> MEEPEEPADSGQSLVPVYIYSPEYVSMCDSLAKIPKRASMVHSLIEAYALHKQMRIVKPKVASMEEMATFHTDAYLQHLQKVSQEGDDDHLDSIEYGLGYDCPATEGIFDYAAAIGGAT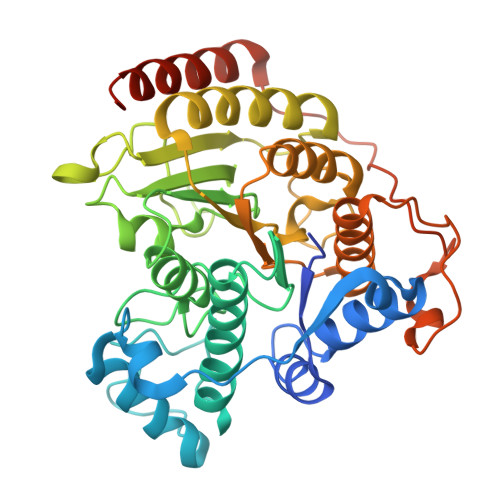ITAAQCLIDGMCKVAINWSGGWHHAKKDEASGFCYLNDAVLGILRLRRKFERILYVDLDLHHGDGVEDAFSFTSKVMTVSLHKFSPGFFPGTGDVSDVGLGKGRYYSVNVPIQDGIQDEKYYQICESVLKEVYQAFNPKAVVLQLGADTIAGDPMCSFNMTPVGIGKCLKYILQWQLATLILGGGGFNLANTARCWTYLTGVILGKTLSSEIPDHEFFTAYGPDYVLEITPSCRPDRNEPHRIQQILNYIKGNLKHVVIEGRGSHHHHHH> MENTENSVD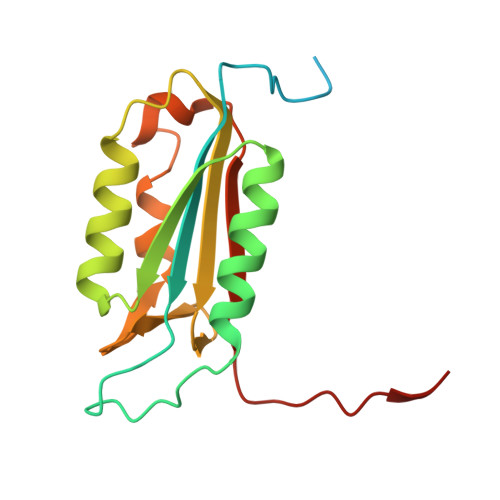SKSIKNLEPKIIHGSESMDSGISLDNSYKMDYPEMGLCIIINNKNFHKSTGMTSRSGTDVDAANLRETFRNLKYEVRNKNDLTREEIVELMRDVSKEDHSKRSSFVCVLLSHGEEGIIFGTNGPVDLKKITNFFRGDRCRSLDGKPKLFIIQACRGTELDCGIETD> SGSMEIRVRVEK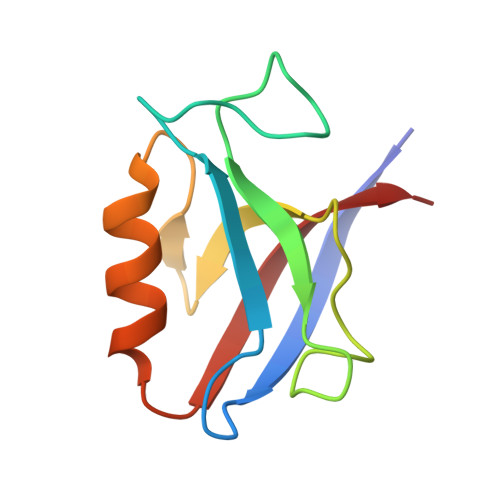DPEIGFRIAGGVGGRGNPFRPDDDGIFVTRVSPEGPASKLLQPGDKIIQANGYSFINIELGQAISLLKTFQNTVELIIVREV>[7x]MTLVPYVVEDTGRGERAMDIYSRLLKDRIVMIGQEIT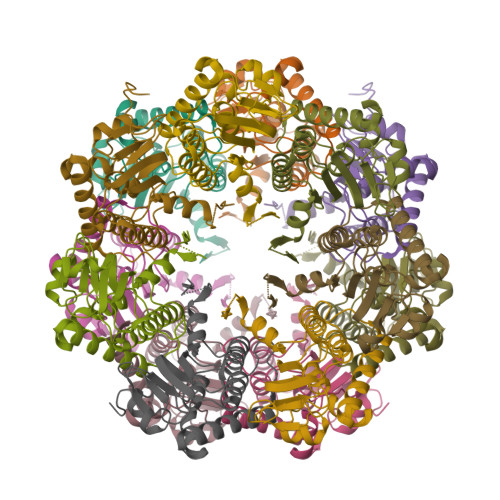EPLANTVIAQLLFLMSEDPTKDIQIFINSPGGYITAGLAIYDTIRFLGCDVNTYCIGQAASMGALLLSAGTKGKRYALPHSRMMIHQPSGGIIGTSADIQLQAAEILTLKKHLSNILAECTGQSVEKIIEDSERDFFMGAEEAIAYGLIDKVISSAKETKDKSIAS> SNAMQIKELAELTGVSVRTLHHYDKIGLLVPQKDDWNGYRIYSEKDVDKLQQILFFKELDFP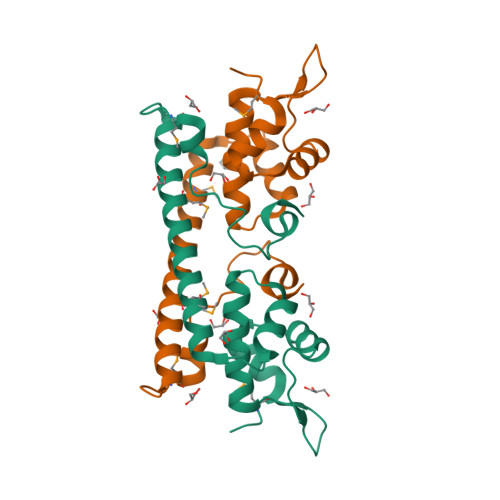LKKIQQILDDPLFDKNVALDMQRHLLIEKKQRIETMLATLDLTIKNEKGEITMTNKEKFTGFDFSSNPYEEEARKLWGDKVVEKANEKVNNMSEKEQLTLKESFDAEFRHLASVRKLTPESEEAQLEIDHFFHYLNDTHGNIYSLEAFASLGEMYVNDERFTKNIDQFGDGLSQFLQEAMTIYAKNK4-(diethylamino)benzaldehyde 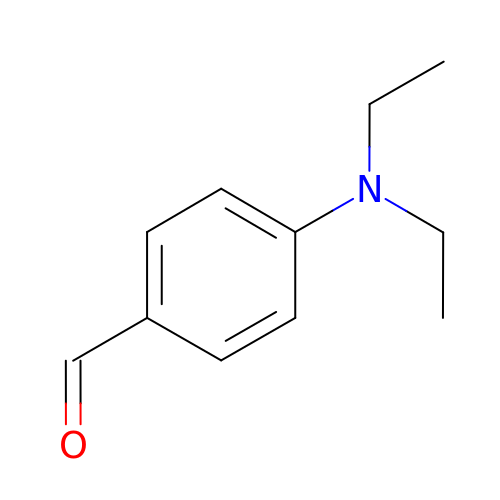| C11 H15 N O | MNFZZNNFORDXSV-UHFFFAOYSA-N>[2x]VPAARSEDRYRNPKGSACSR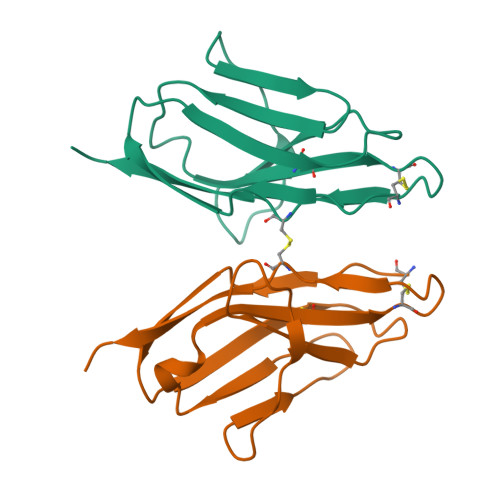IWQSPRFIARKRGFTVKMHCYMNSASGNVSWLWKQEMDENPQQLKLEKGRMEESQNESLATLTIQGIRFEDNGIYFCQQKCNNTSEVYQGCGTELRVMGFSTLAQLKQRNTLKD>[6x]KTDITSTKNELVITYHGRLRSFSEEDTYKIKAWLE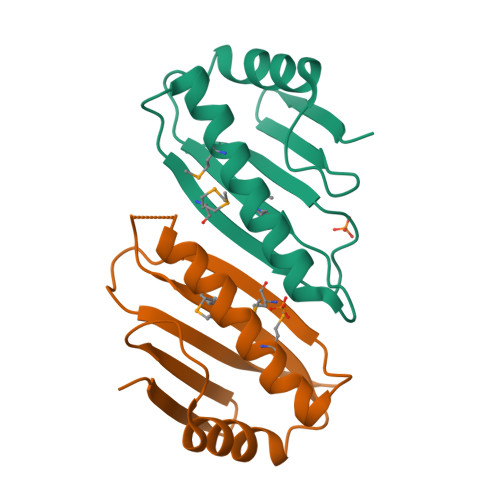DKINSNLLIEMVIPQADISFSDSLRLGYERGIILMKEIKKIYPDVVIDMSVNSAASSTTSKAIITTINK>[3x]VLFEEIRSLLPQKYPFIFIDRAIEFEESKRIVCVKNISGNEPVFVGHFPDFAIMPGVLIIEAMAQASIIL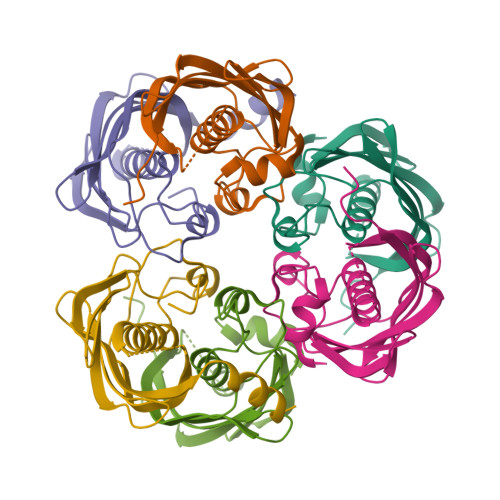FRKSLPSRNDEDAVFLLASVNNARFTKPVVPGDQLTIEVIVEKIVSRGAIVQSVVKVQEKVVAKAALTFGIVEKSSLVLEHHHHHH>MTKKVAIILANEFEDIEYSSPKEALENAGFNTVVIGDTANSEVVGKHGEKVTVDVGIAEAKPEDYDALLIPGGFSPDHLRGDTEGRYGTFAKYFTKNDVPTFAIDHGPQILIDTDDLKGRTLTAVLNVRKDL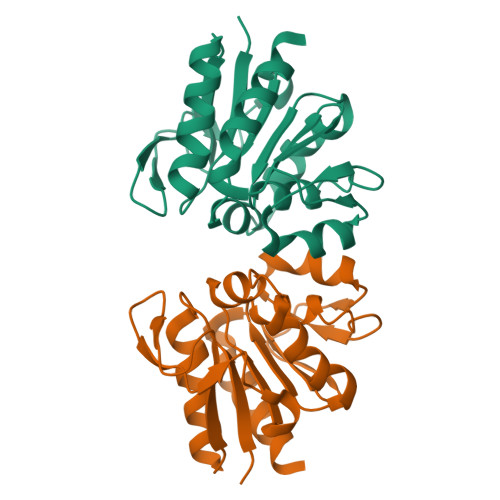SNAGAHVVDESVVVDNNIVTSRVPDDLDDFNREIVKQLQLEHHHHHH[2x]~{N}2-(3-morpholin-4-ylpropyl)pyrido[3,4-g]quinazoline-2,10-diamine 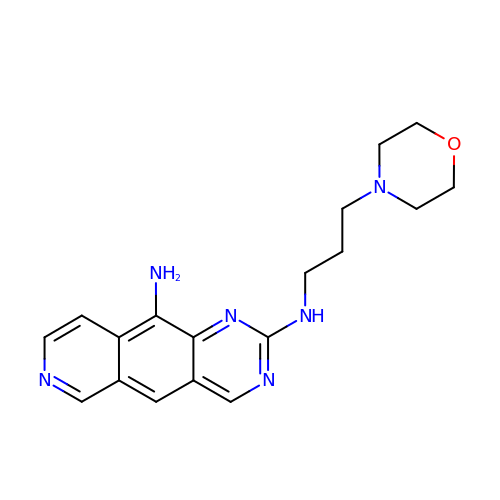| C18 H22 N6 O | LRBZZLHCFITOFC-UHFFFAOYSA-N>GAMANNTIYDFIGIGIGPFNLGLACLSEPVEGLNGVFLDQNPGFDWHTGMMLESAHLQTPFMADLVTLADPTSPYSLLNFMKQKGKLYSFYIREDFFLMRKEYNQYCQWAAERLGNLRWNTRVEYVSYDDNLQCYRVRSTDTVSGKQQEWLAHRLVLGTGPSAWSPACSQPYRERFVHSSEYLLNKEKLQKKRSITVLGSGQSAAEIYYDLLTDIDRFGYQLNWITRAPRFYPLEYTKLTLEMTSPEWIDYFHSLPAAKRDELNASQKNLYKGINSSLINAIYDLLYVKQLDGKLDVNLFTHSELTDMRWLAEGEFELKLHQQEQDRAYSRRTEGLVMATGYHYQPPAFVEGIQQRIQWDEKDRYDVQRNYSIDRHNQVFVQNAELHTHGFVTPDLG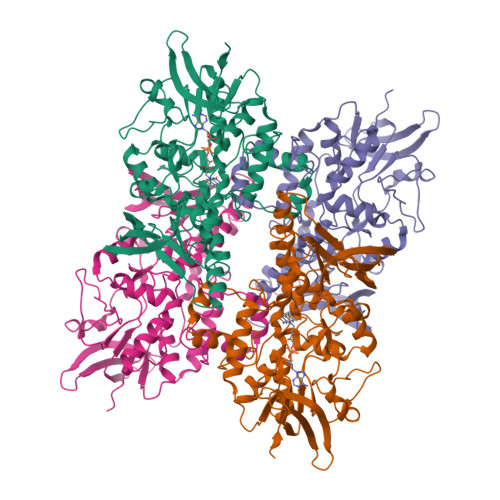MACYRNSVLLREITGREVYPVERQIAFQTFPAQSEM[2x]>SWNKKNEEKEDFGIIVILWKQVTVKEDGKVPLEPFLTAAKEVLRVVDAFGSGFRIVKNDIAGNIKKLYRANQTVHAETLQELIIAENSPDGLATVALLWLKRAFQFIASFLRRLVVTDKSLEQCVTEAYNCTLRPCHSAVIQKVFWGGVKLAPSRERFYRKLHPDLNIAKAKIEEFLIELHDPLCCIVQFFFQRELEDQCWGDEVYQRKDSSE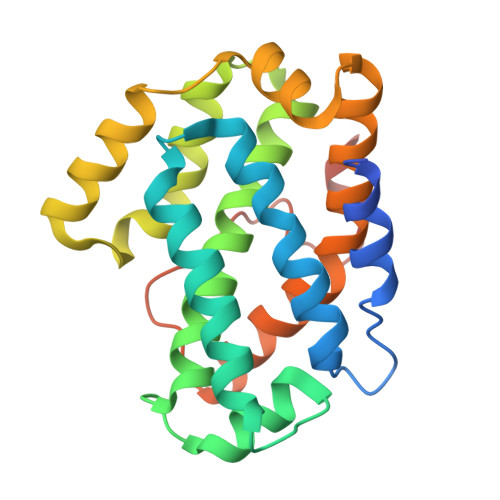WLKVSCEQDSV[2x]> GIVNVPNPNNTKFQELARFAIQDYNKKQNAHLEFVENLNVKEQVVAGIMYYITLAATDDAGKKKIYKAKIWVKEWEDFKKVVE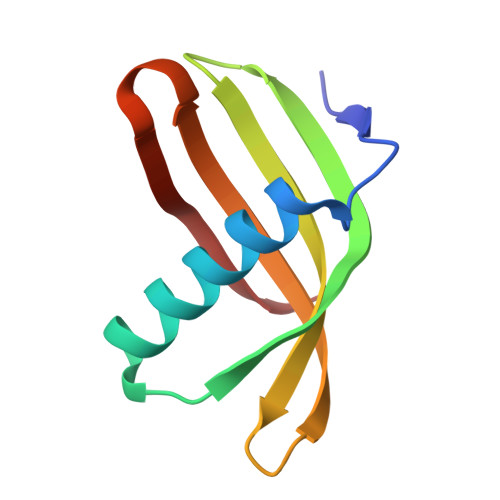FKLV> NDDDVQKAD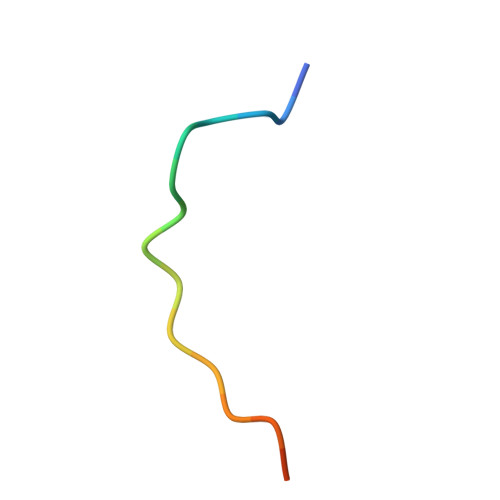VSSTGQGV> GHMAVPDDDDDDDNSNDESEYESSQMDSEKNKGSIKNSKNVVIYADGVYDMLHLGHMKQLEQAKKLFENTTLIVGVTSDNETKLFKGQVVQTLEERT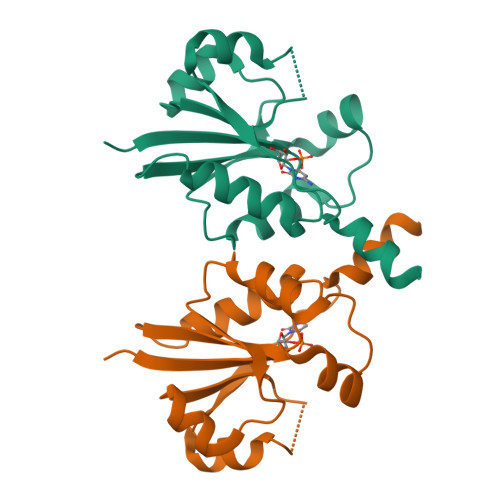ETLKHIRWVDEIISPCPWVVTPEFLEKYKIDYVAHDDIPYANNQKEDIYAWLKRAGKFKATQRTEGVSTTDLIVRILKNYEDY By integrating structure‐informed design, crystallography, and machine learning‐augmented all‐atom molecular dynamics simulations (MD), we synthesized, biophysically and biochemically characterized, and studied the dissociation of a library of small molecule activators of the 5‐aminoimidazole–4–carboxamide ribonucleotide triphosphate (ZTP) riboswitch, a ligand‐binding RNA motif that regulates bacterial gene expression. Riboswitches control gene expression by sensing the intracellular concentration of a cognate ligand and, upon binding, undergo a conformational change that regulates gene expression. The ZTP riboswitch undergoes a ligand‐gated competitive strand displacement to form the terminator hairpin during transcription, and the binding of ZMP stabilizes the pseudoknot, disfavoring terminator hairpin formation. Further, we established that ligand on‐rates determine activation potency as opposed to binding affinity and elucidated RNA structural differences, which provide mechanistic insights into the interplay of RNA structure on riboswitch activation.

Previously, isosteric replacement of the phosphate and ribose sugar moiety of ZMP with a pyridine group resulted in the discovery of compound 1. Compound 1 possessed a weaker affinity (K D ∼600 nM) but was a stronger riboswitch activator (T 50 ∼5.8 µM) than cognate ligand ZMP (K D ∼324 nM and T 50 ∼37 µM) in biochemical assays. Our previously reported structure of compound 1 was determined at 3.2 Å resolution bound to the F. ulcerans ZTP riboswitch; thus, we sought to validate those findings in the S. odontolytica ZTP riboswitch, which has been reported to crystallize at higher resolution. We co‐crystallized 1 with the S. ondontolytica ZTP riboswitch aptamer, solved the structure via molecular replacement, and refined the structure to 2.4 Å resolution. In the model, the pyridine moiety is poised to hydrogen bond to the 2'‐OH of G51 (3.0 Å), consistent with our previous findings. Nearby C52 is about 4.0 Å away from the pyridinyl group and hydrogen bonds with non‐bridging phosphate oxygen (NBPO) O2 of C50 (3.0 Å). In the presence of ZMP, a hydrated magnesium ion makes inner sphere contacts with C52. Access to crystal structures of RNA bound to ligands is frequently difficult to acquire, and in this work crystallography was only successful with an aptamer from the S. ondontolytica ZTP aptamer, which has a similar ligand binding site. Although an imperfect comparison, the structural work demonstrates that the new compounds bind via a consistent mode and coordinate to the conserved magnesium ion.

> GGGUCGUGACUGGCGAACAGGUGGGAAACCACCGGGGAGCGACCCUUGCCGCCCGCCUGGGCAA>[3x]YDALSCKLAAISVGYLPSSGLQRLSVDLSKKYTEWHRSYLITLKKFSRRAFGKVDKAMRSSFPVMNYGTYLRTVGIDAAILEFLVANEKVQVVNLGCGSDLRMLPLLQMFPHLAYVDIDYNESVELKNSILRESEILRISLGLSKEDTAKSPFLIDQGRYKLAACDLNDITETTRLLDVCTKREIPTIVISECLLCYMHNNESQLLINTIMSK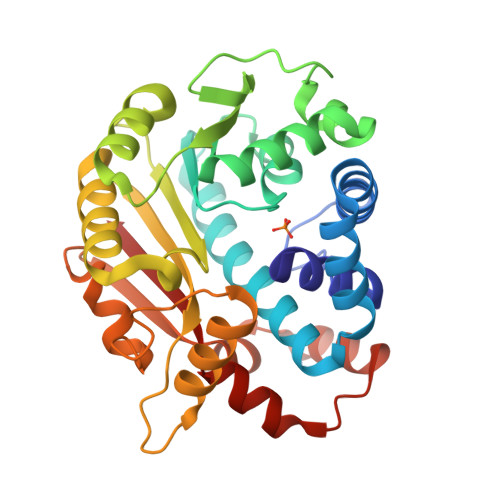FSHGLWISYDPIGGSQPNDRFGAIMQSNLKESRNLEMPTLMTYNSKEKYASRWSAAPNVIVNDMWEIFNAQIPESERKRLRSLQFLDELEELKVMQTHYILMKAQW>[2x]MGGSHHHHHHGMASWSHPQFEKGGHHHHHHGGSGENLYFQGGSGPKFNETADKYLKSGSAEAELIILQYIQQDRVSEDDEEWVYNLLEKANNPYIKLNALLWLSAKRKYLTQLSKLWGISENELKSLSQQQPKIGLFPAVDSRKNAFLAKVFVYKLKSEEPIALAILGDKIENFSYLAQLGKQNCLIGFNKNIQGNSWQLAVLATLLVKDEKIISKIAYSGIVLPSGEIITAEEIEYKKRCCQNLVHRIKKIEQLDAWLNTETIPLPVIQYQGEENELKRWQKAMEQKVQEKFSWFSYELLEDFYGITNSDLAIFGNGILPFEANAWQKLLQEQVKDKFKLLEDKVMPKKVLWFYAGQISTLQLGIGALFGFKRAVSILQMEFSNTTYHEVFILYGKENARQLKNVSVKKEDYQYIQSELLINEPHKNELGFIIYLGSHNPIGEAKAYCQKQLQINNFLIIQARENQ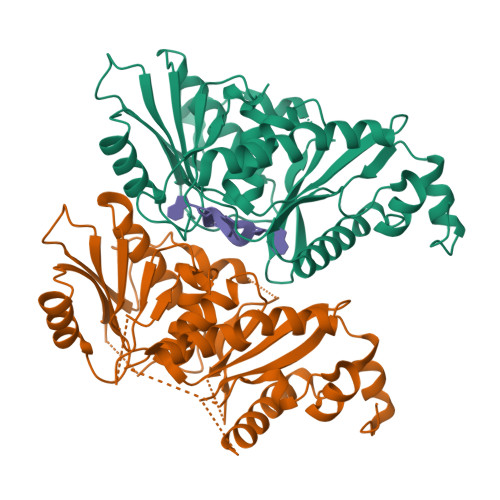GVMETSQNWLPYLQEINSALNTARQEYHWERIHLFQTAPTALCMALGIAVGHFLPVDVYHYQFNAEEPKYRCVFSLDKMLNL> MSRPLSDQEKRKQISVRGLAGVENVTELKKNFNRHLHFTLVKDRNVATPRDYYFALAHTVRDHLVGRWIRTQQHYYEKDPKRIYYLSLEFYMGRTLQNTMVNLALENACDEATYQLGLDMEELEEIEEDAGLGNGGLGRLAACFLDSMATLGLAAYGYGIRYEFGIFNQKICGGWQMEEADDWLRYGNPWEKARPEFTLPVHFYGRVEHTSQGAKWVDTQVVLAMPYDTPVPGYRNNVVNTMRLWSAKAPNDFNLKDFNVGGYIQAVLDRNLAENISRVLYPNDNFFEGKELRLKQEYFVVAATLQDIIRRFKSSKFGCRDPVRTNFDAFPDKVAIQLNDTHPSLAIPELMRVLVDLERLDWDKAWEVTVKTCAYTNHTVLPEALERWPVHLLETLLPRHLQIIYEINQRFLNRVAAAFPGDVDRLRRMSLVEEGAVKRINMAHLCIAGSHAVNGVARIHSEILKKTIFKDFYELEPHKFQNKTNGITPRRWLVLCNPGLAEIIAERIGEEYISDLDQLRKLLSYVDDEAFIRDVAKVKQENKLKFAAYLEREYKVHINPNSLFDVQVKRIHEYKRQLLNCLHVITLYNRIKKEPNKFVVPRTVMIGGKAAPGYHMAKMIIKLITAIGDVVNHDPVVGDRLRVIFLENYRVSLAEKVIPAADLSEQISTAGTEASGTGNMKFMLNGALTIGTMDGANVEMAEEAGEE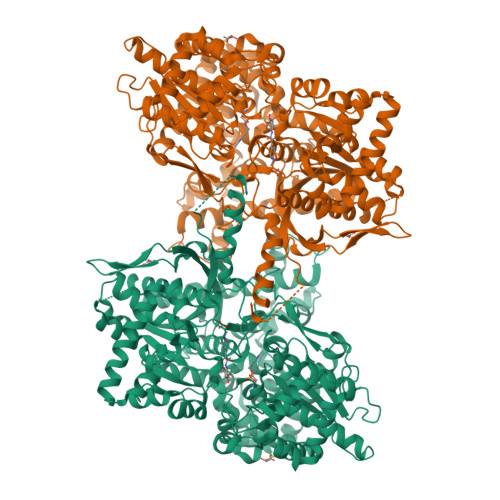NFFIFGMRVEDVDRLDQRGYNAQEYYDRIPELRQIIEQLSSGFFSPKQPDLFKDIVNMLMHHDRFKVFADYEEYVKCQERVSALYKNPREWTRMVIRNIATSGKFSSDRTIAQYAREIWGVEPSRQRLPAPDEKIP>KHSLPDLPYDYGALEPHINAQIMQLHHSKHHAAYVNNLNVTEEKYQEALAKGDVTAQIALQPALKFNGGGHINHSIFWTNLSPNGGGEPKGELLEAIKRDFGSFDKFKEKLTAASVGVQGSGWGWLGFNKERGHLQIAACPNQDPLQGTTGLIPLLGIDVWEHAYYLQYKNVRPDYLKAIWNVINWENVTE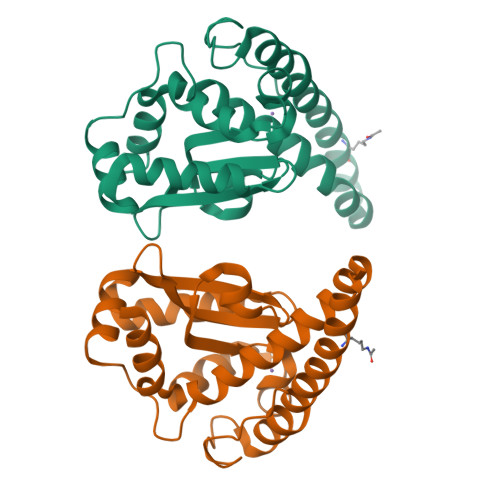RYMACKK[2x]> MFCFQCQETAKNTGCTVKGMCGKPEETANLQDLLIFVLRGIAIYGEKLKELGQPDRSNDDFVLQGLFATITNANWDDARFEAMISEGLARRDKLRNAFLAVYKAKNGKDFSEPLPEAATWTGDSTAFAEKAKSVGILATENEDVRSLRELLIIGLKGVAAYAEHAAVLGFRKTEIDEFMLEALASTTKDLSVDEMVALVMKGRRMAVTTMALLDEANTTTYGNPEITQVNIGVGKNPGILISGHDLKDMAELLKQTEGTGVDVYTHGEMLPANYYPAFKKYPHFVGNYGGSWWQQNPEFESFNGPILLTTNCLVPLKKENTYLDRLYTTGVVGYEGAKHIADRPA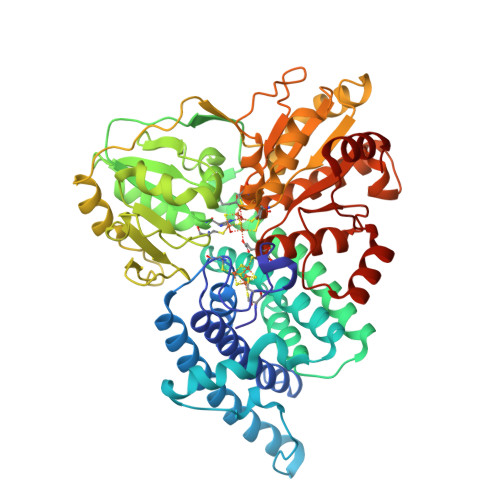GGAKDFSALIAQAKKCPPPVEIETGSIVGGFAHHQVLALADKVVEAVKSGAIKRFVVMAGCDGRQKSRSYYTEVAENLPKDTVILTAGCAKYRYNKLNLGDIGGIPRVLDAGQCNDSYSLAVIALKLKEVFGLDDINDLPVSYDIAWYEQKAVAVLLALLFLGVKGIRLGPTLPAFLSPNVAKVLVENFNIKPIGTVQDDIAAMMAGK>[4x]GADLISMKGDVITEHQFYEQVKNNPSAQQVLLNMTIQKVFEKQYGSELDDKEVDDTIAEEKKQYGENYQRVLSQAGMTLETRKAQIRTSKLVELAVKKVAEAELTDEAYKKAFDEYTPDVTAQIIRLNNEDKAKEVLEKAKAEGADFAQLAKDNSTDEKTKENGGEITFDSASTEVPEQVKKAAFALDVDGVSDVIT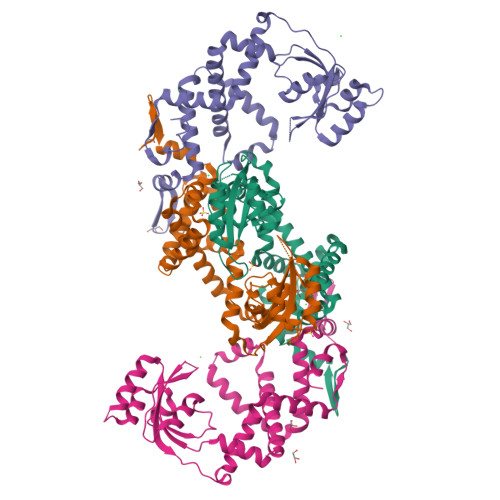ATGTQAYSSQYYIVKLTKKTEKSSNIDDYKEKLKTVILTQKQNDSTFVQSIIGKELQAANIKVKDQAFQNIFTQYIGGGDSSSSSSTSNE> MASHMLSWLHEINSQELEKAHATLLGLANMETRYFAKKKTLLGLSKLAALASDFSEDMLQEKIEEMAEQERFLLHQETLPEQLLAEKQLNLSAMPVLTAPQLIGLYICEENRRANEYDFKKALDLLEYIDEEEDININDLKLEILCKALQRDNWSSSDGKDDPIEVSKDSI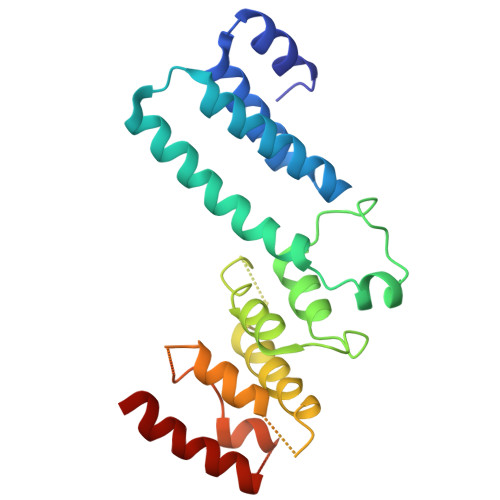FVKILQKLLKDGIQLSEYLPEVKDLLQADQLGSLKSNPYFEFVLKANYEYYVQGQI>SSLKPFTYPFPETRFLHAGPNVYKFKIRYGKSIRGEEIENKEVITQELEDSVRVVLGNLDNLQPFATEHFIVFPYKSKWERVSHLKFKHGEIILIPYPFVFTLYVEMKW[3x];>TGYISIDAMKKFLGELHDFIPGTSGYLAYH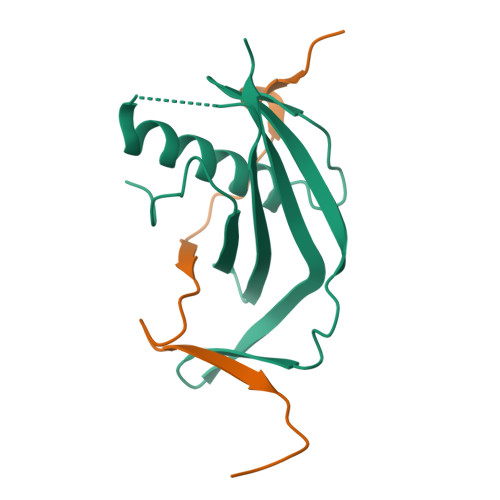VQNEIN[3x]> GMDNVAEYRKLIKQVLTEYDNLSRQSPETNYETCLVFDENHDNYLWLAVDWQGSKRIKYTYVHIRIKNEKIYIEEDYTEEGIATELMRLGVTNNDIVLAF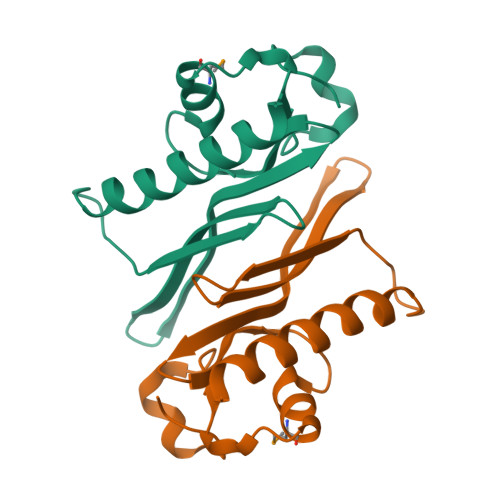HPPDVRKFTDFATA>GIKCFAVRSLGWVEMTEEELAPGRSSVAVNNCIRQLSYHKNNLHDPMSGGWGEGKDLLLQLEDETLKLVEPQSQALLHAQPIIS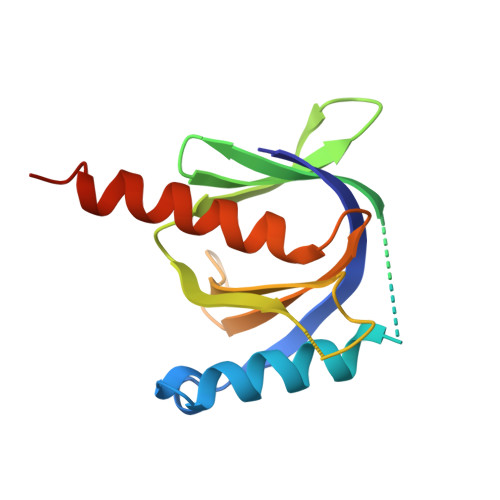IRVWGVGRDSGRERDFAYVARDKLTQMLKCHVFRCEAPAKNIATSLHEICSKIMAELEHHHHHH[4x]>[4x]MHHHHHHLPNITILATGGTIAGGGDSATKSNYTVGKVGVENLVNAVPQLKDIANVKGEQVVNIGSQDMNDNVWLTLAKKINTDCDKTDGFVITHGTDTMEETAYFLDLTVKCDKPVVMVGAMRPSTSMSADGPFNLYNAVVTAADKASANRGVLVVMNDTVLDGRDVTKTNTTDVATFKSVNYGPLGYIHNGKIDYQRTPARKHTSDTPFDVSKL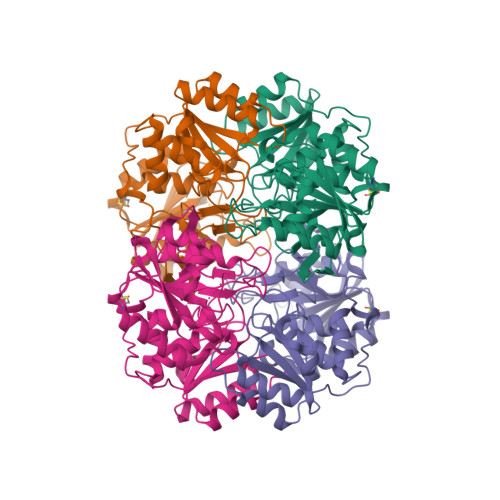NELPKVGIVYNYANASDLPAKALVDAGYDGIVSAGVGNGNLYKSVFDTLATAAKTGTAVVRSSRVPTGATTQDAEVDDAKYGFVASGTLNPQKARVLLQLALTQTKDPQQIQQIFNQY> APLAYERPVLHLVALNTPVAGDIRADFQCFQQARAAGLLSTFRAFLSSHLQDLSTVVRKAERFGLPIVNLKGQVLFNNWDSIFSGDGGQFNTHIPIYSFDGRDVMTDPSWPQKVVWHGSNPHGVRLVDKYCEAWRTTDMAVTGFASPLSTGKILDQKAYSCANRLIVLCIENS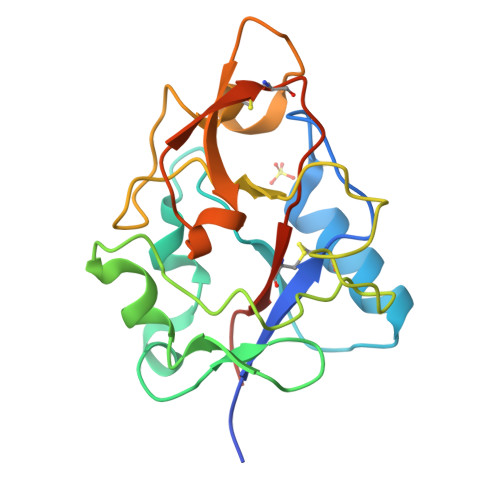FMTDTRK> TVAYIAIGSALASPLEQVNAALKALGDIPESHILTVSSFYRTPPLGPQDQPDYLNAAVALETSLAPEELLNHTQRIELQQGRVRKAERWGPRTLDLDIMLFGNEVINTERLTVPHYDMKNRGFM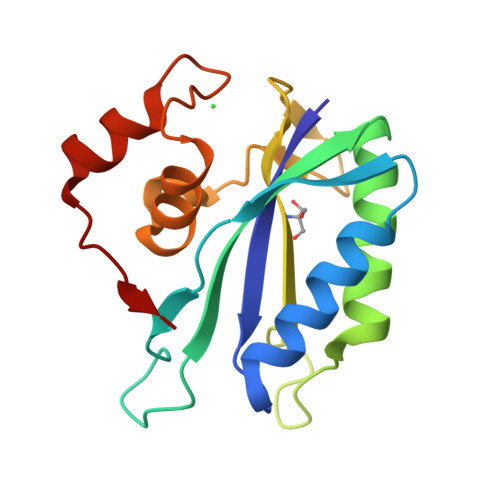LWPLFEIAPELVFPDGEMLRQILHTRAFDKLNKW> VTKTIPVTVKANPVLETIAVDSTGVSVAKGQKATFKVTLKDQYGNKFTGNVNVTSDKTETATVSVSNSGIGQSEYTVTVNGVAEGSTTITIKSGTKEVKVPVNVVAGGPVANYQIKVLDDGKIDKSATESPANNDVQLKVYAVDANGNIVGDITNDVTITSEATDTNGVIVNASKS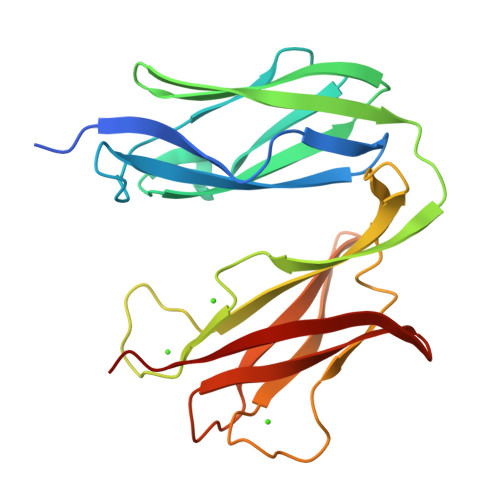TANGDTVYVITDNGSKKVGKETLTVKLGTVTLGTVDVEVIDTT> MAEQTLLSKLNALSQKVIPPASPSQASILTEEVIRNWPERSKTLCSDFTALESNDEKEDWLRTLFIELFDFINKNDENSPLKLSDVASFTNELVNHERQVSQASIVGKMFIAVSSTVPNINDLTTISLCKLIPSLHEELFKFSWISSKLLNKEQTTLLRHLLKKSKYELKKYNLLVENSVGYGQLVALLILAYYDPDNFSKVSAYLKEIYHIMGKYSLDSIRTLDVILNVSSQFITEGYKFFIALLRKSDSWPSSHVANNSNYSSLNEGGNMIAANIISFNLSQYNEEVDKENYERYMDMCCILLKNGFVNFYSIWDNVKPEMEFLQEYIQNLETELEEESTKGVENPLAMAAALSTENETDEDNALVVNDDVNMKDKISEETNADIESKGKQKTQQDILLFGKIKLLERLLIHGCVIPVIHVLKQYPKVLYVSESLSRYLGRVFEYLLNPLYTSMTSSGESKDMATALMITRIDNGILAHKPRLIHKYKTHEPFESLELNSSYVFYYSEWNSNLTPFASVNDLFENSHIYLSIIGPYLGRIPTLLSKISRIGVADIQKNHGSESLHVTIDKWIDYVRKFIFPATSLLQNNPIATSEVYELMKFFPFEKRYFIYNEMMTKLSQDILPLKVSFNKAEREAKSILKALSIDTIAKESRRFAKLISTNPLASLVPAVKQIENYDKVSELVVYTTKYFNDFAYDVLQFVLLLRLTYNRPAVQFDGVNQAMWVQRLSIFIAGLAKNCPNMDISNIITYILKTLHNGNIIAVSILKELIITVGGIRDLNEVNMKQLLMLNSGSPLKQYARHLIYDFRDDNSVISSRLTSFFTDQSAISEIILLLYTLNLKANTQNSHYKILSTRCDEMNTLLWSFIELIKHCLKGKAFEENVLPFVELNNRFHLSTPWTFHIWRDYLDNQLNSNENFSIDELIEGAEFSDVDLTKISKDLFTTFWRLSLYDIHFDKSLYDERKNALSGENTGHMSNRKKHLIQNQIKDILVTGISHQRAFKKTSEFISEKSNVWNKDCGEDQIKIFLQNCVVPRVLFSPSDALFSSFFIFMAFRTENLMSILNTCITSNILKTLLFCCTSSEAGNLGLFFTDVLKKLEKMRLNGDFNDQASRKLYEWHSVITEQVIDLLSEKNYMSIRNGIEFMKHVTSVFPVVKAHIQLVYTTLEENLINEEREDIKLPSSALIGHLKARLKDALELDEFCTLTEEEAEQKRIREMELEEIKNYETACQNEQKQVALRKQLELNKSQRLQNDPPKSVASGSAGLNSKDRYTYSRNEPVIPTKPSSSQWSYSKVTRHVDDINHYLATNHLQKAISLVEND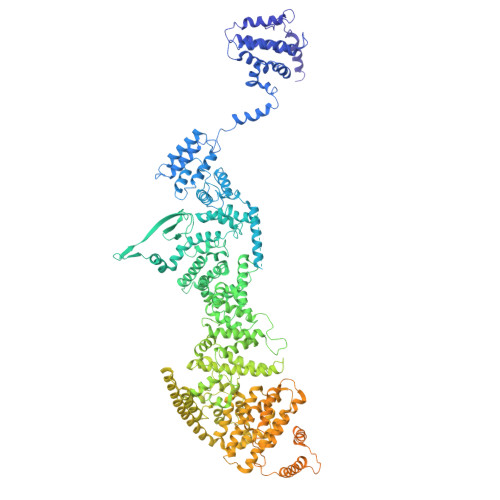DETRNLRKLSKQNMPIFDFRNSTLEIFERYFRTLIQNPQNPDFAEKIDSLKRYIKNISREPYPDTTSSYSEAAAPEYTKRSSRYSGNAGGKDGYGSSNYRGPSNDRSAPKNIKPISSYAHKRSELPTRPSKSKTYNDRSRALRPTGPDRGDGFDQRDNRLREEYKKNSSQRSQLRFPEKPFQEGKDSSKANPYQASSYKRDSPSENEEKPNKRFKKDETIRNKFQTQDYRNTRDSGAAHRANENQRYNGNRKSNTQALPQGPKGGNYVSRYQR>MSPLAQNGGGTAGTTGLRNNCDGSTFVPVTGSAGNAPSKWDCQLLRDGYIAKQNKSWLISGPRI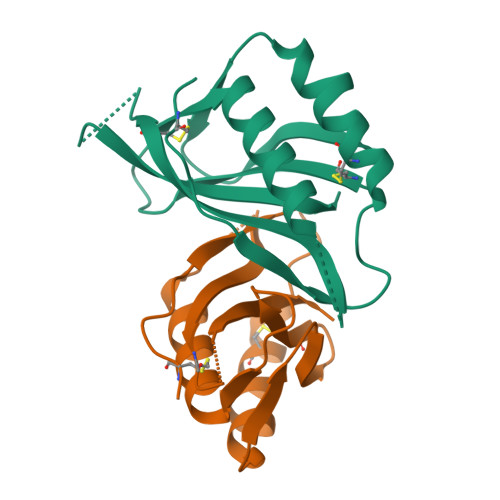IGTVRTCQFSATVDVSGTAGWIGRDDIMDLMKDSLNLWKDGETTQVQGAMQVGESGDVNCVAGKKGEGQKVRIAWTLGHS[8x]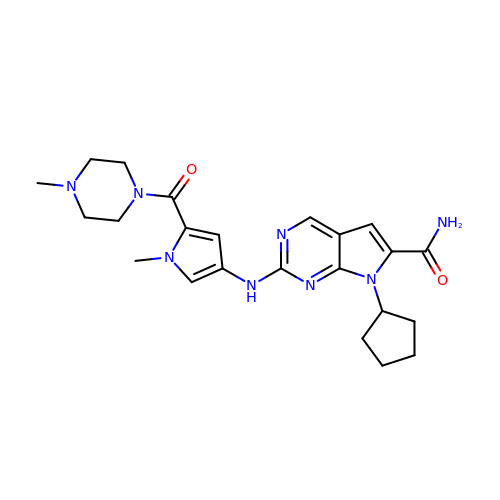7-cyclopentyl-2-({1-methyl-5-[(4-methylpiperazin-1-yl)carbonyl]-1H-pyrrol-3-yl}amino)-7H-pyrrolo[2,3-d]pyrimidine-6-carboxamide | C23 H30 N8 O2 | CXCXNZWXDOVZBA-UHFFFAOYSA-N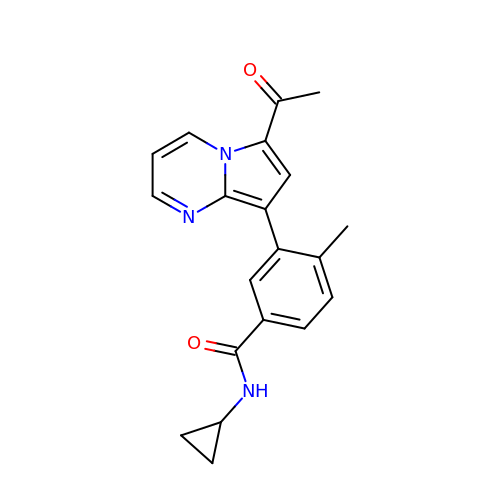3-(6-acetylpyrrolo[1,2-a]pyrimidin-8-yl)-N-cyclopropyl-4-methylbenzamide | C20 H19 N3 O2 | RPBMXJHQYJLPDN-UHFFFAOYSA-N> MEEPEEPADSGQSLVPVYIYSPEYVSMCDSLAKIPKRASMVHSLIEAYALHKQMRIVKPKVASMEEMATFHTDAYLQHLQKVSQEGDDDHPDSIEYGLGYDCPATEGIFDYAAAIGGATITAAQCLIDGMCKVAINWSGGWHHAKKDEASGFCYLNDAVLGILRLRRKFERILYVDLDLHHGDGVEDTFSFTSKVMTVSLHKFSPGFFPGTGDVSDVGLGKGRYYSVNVPIQDGIQDEKYYQICESV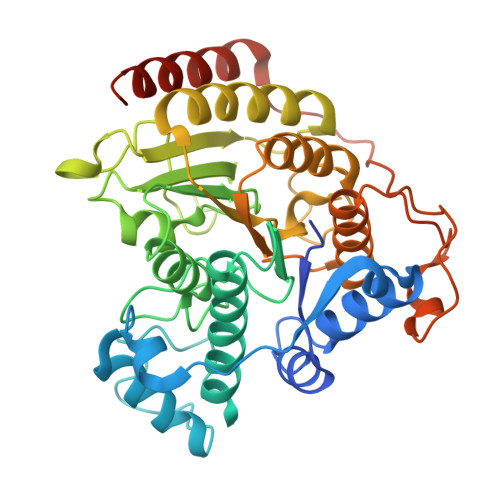LKEVYQAFNPKAVVLQLGADTIAGDPMCSFNMTPVGIGKCLKYILQWQLATLILGGGGFNLANTARCWTYLTGVILGKTLSSEIPDHEFFTAYGPDYVLEITPSCRPDRNEPHRIQQILNYIKGNLKHVVIEGRGSHHHHHH(2R)-sulfonatepropionyl-amino(dethia)-CoA | C24 H41 N8 O20 P3 S 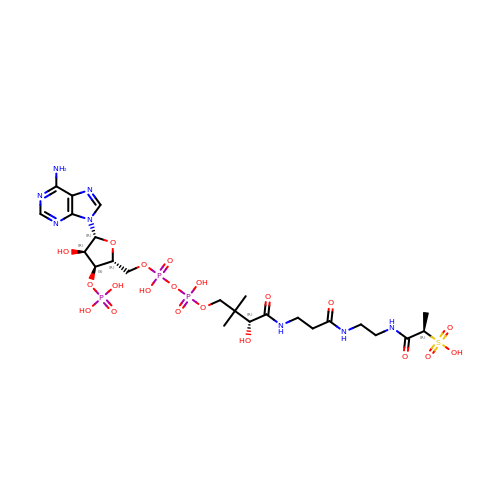| IUFNAUQYWOGJPI-AMWHPSEWSA-N> MGSDKIHHHHHHMIRLGLTSFSEHDYLTGKKRSTLYEYASHLPLVEMDTAYYGIPPKERVAEWVKAVPENFRFVMKVYSGISCQGEWQTYYASEEEMITAFLESMAPLIESKKLFAFLVQFSGTFGCTKENVAYLQKIRHWFKDLPIAIELRNN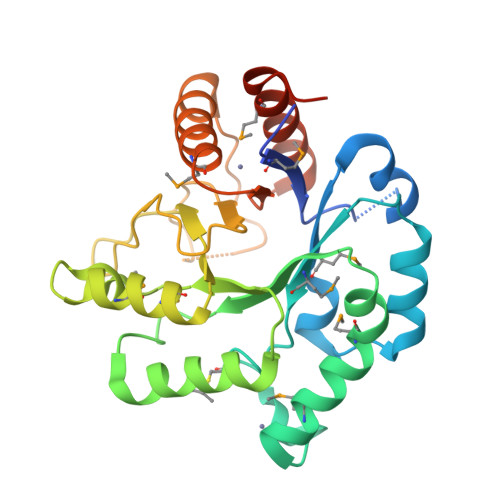SWYQPNFVKQMLQFMKENQFSLVIVDEPQIPTNPVPFYPYVTNPNLVLFRFHGRNAAGWLANDAEWRKKRTLYHYNTQEIADLSEAVLKMSQEAKEVGVIFNNNSGGDAAENALQMQKVLNLSYDDLNPKQLDLF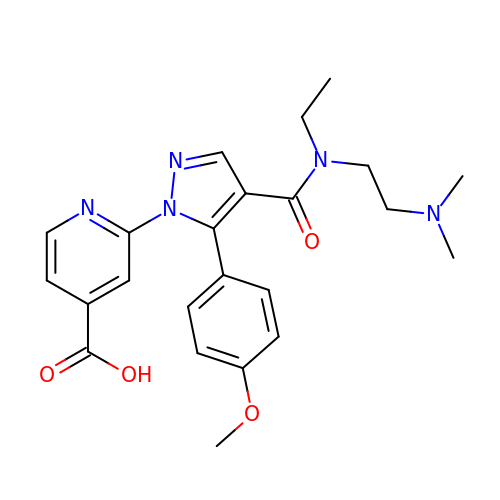2-[4-{[2-(dimethylamino)ethyl](ethyl)carbamoyl}-5-(4-methoxyphenyl)-1H-pyrazol-1-yl]pyridine-4-carboxylic acid | C23 H27 N5 O4 | ICCHWGKLRKRQKD-UHFFFAOYSA-N> NCCVKGNSIYPQKTSTKQTGLMLDIARHFYSPEVIKSFIDTISLSGGNFLHLHFSDHENYAIESHLLNQRAENAVQGKDGIYINPYTGKPFLSYRQLDDIKAYAKAKGIELIPELDSPNHMTAIFKLVQKDRGVKYLQGLKSRQVDDEIDITN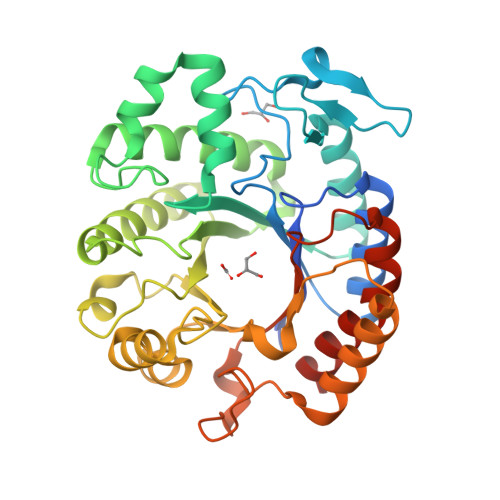ADSITFMQSLMSEVIDIFGDTSQHFHIGGDEFGYSVESNHEFITYANKLSYFLEKKGLKTRMWNDGLIKNTFEQINPNIEITYWSYDGDTQDKNEAAERRDMRVSLPELLAKGFTVLNYNSYYLYIVPKASPTFSQDAAFAAKDVIKNWDLGVWDGRNTKNRVQNTHEIAGAALSIWGEDAKALKDETIQKNTKSLLEAVIHKTNGDEHHHHHH> MDPAHHIKDTS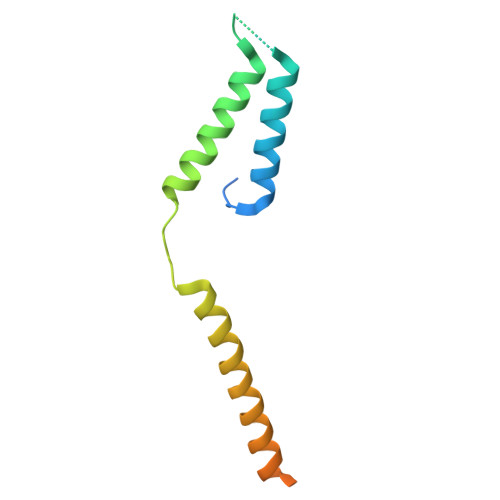AELLSQQDFSILQSRLLEFLASQEARETVTASKELTLLRQGIRQLKEKVSKMEPEEMTVKEKKSIIEILKARIALKKAFLKMALSESNDTVVKKEDVRESPVDTFMENAT>NNUNANN[2x];>GGU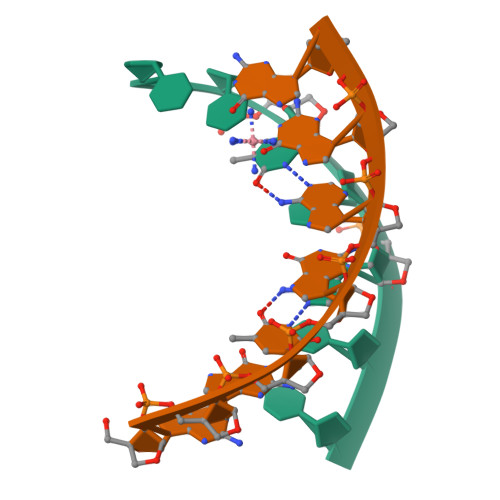GAGG[2x]>[3x]MSIEKLKAALPEYAKDIKLNLSSITRSSVLDQEQL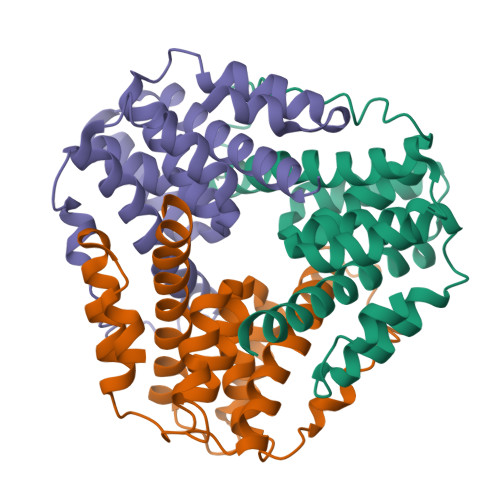WGTLLASAAATRNPQVLADIGAEATDHLSAAARHAALGAAAIMGMNNVFYRGRGFLEGRYDDLRPGLRMNIIANPGIPKANFELWSFAVSAINGCSQCLVAHEHTLRTVGVDREAIFEALKAAAIVSGVAQALATIEALSPS> KSAVT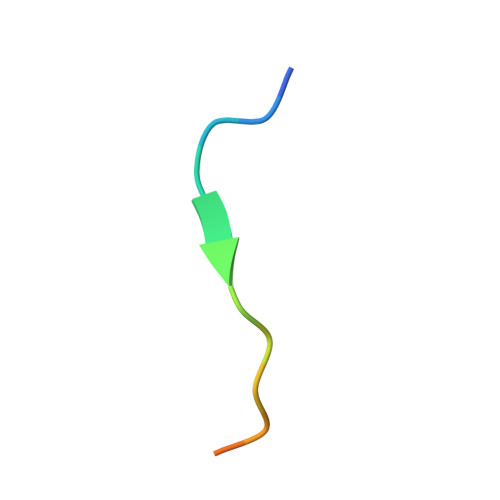TVVNPKYEGK>GHAEIMPPPPKPKDRTIPIPISKPPVFIGKDRTEPVKGFHKAMVKTMSAALKIPHFGYCDEVDLTELVKLREELKPIAFARGIKLSFMPFFLKAASLGLLQFPILNASVDENCQNITYKASHNIGIAMDTEQGLIVPNVKNVQIRSIFEIATELNRLQKLGSAGQLSTNDLIGGTFTLSNIGSIGGTYAKPVILPPEVAIGALGTIKALPRFNEKGEVCKAQIMNVSWSADHRIIDGATVSRFSNLWKSYLENPAF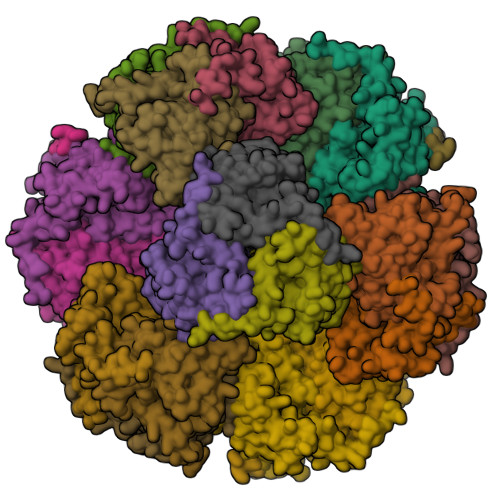MLLDLK[8x]>AECSVDIQGNDQMQFNTNAITVDKSCKQFTVNLSHPGNLPKN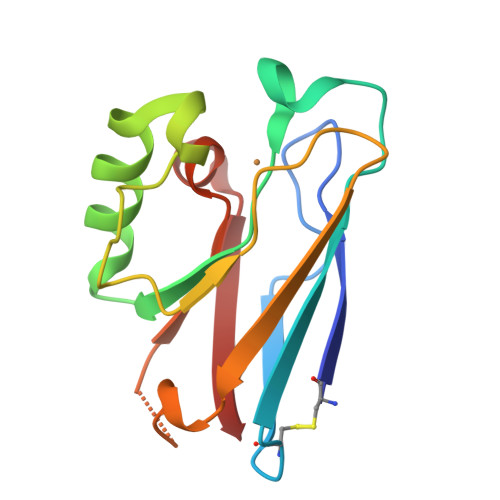VMGHNWVLSTAADMQGVVTDGMASGLDKDYLKPDDSRVIAHTKLIGSGEKDSVTFDVSKLKEGEQYMFFCSPHQGAGMKGTLTLK[2x]>[2x]GSHMANLDRTDDLVYLNVMELVRAVLELKNELSQLPPEGYVVVVKNVGLTLRKLIGSVDDLLPSLPSSSRTEIEGTQKLLNKDLAELINKMR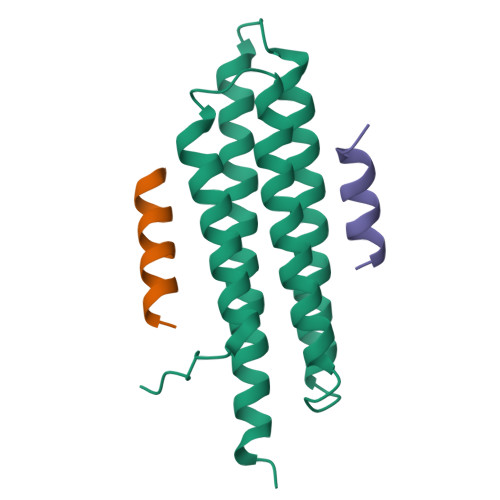LAQQNAVTSLSEEAKRQMLTASHTLAVDAKNLLDAVDQAKVLANLAH;>MEELDALLEELERSTLQDSD[4x]Cytochrome P450 monooxygenases (CYPs) constitute a superfamily of heme-containing enzymes that are widely distributed among all biological kingdoms; they catalyze the hydroxylation of a wide variety of substrate molecules. CYP105s are the only CYP family that have been conserved with representatives in every Streptomyces species thus far investigated. Finally, we verified that CYP105P2 is a bacterial flavone hydroxylase, with potential for use as a biocatalyst. Our sequence analysis showed that CYP105P2 shares a high identity (92%) with CYP105P1 from S. avermitilis, and that it contains a dioxygen-binding region and a heme-iron-binding region, both of which are typical motifs of CYPs.

The structure of CYP105P2 from S. peucetius was determined at a resolution of 2.1 Å. It contains 15 α-helices and six β-strands. The putative active site of CYP105P2 is composed of a heme group and hydrophobic substrate-binding site. Although no exogenous ligands were added to the CYP105P2 protein during purification or crystallization, initial experimental maps indicated the presence of an unknown ligand near the active sites of both molecules in the asymmetric unit. A careful examination of the (Fo − Fc) difference density map following refinement indicated that there was a distinct electron density with a bent V-shape. The conformation of this density suggests that it could be interpreted as a biphenyl derivative, which was then fitted into this electron density map. A ligand resembling the biphenyl compound bisphenol A was unexpectedly found in the substrate-binding cavity; this ligand was probably incorporated during protein expression in E. coli. The bound ligand forms strong hydrophobic interactions with Pro82, Ala181, Met187, Leu189, Leu193, and Ile236 side-chains. In addition, the hydroxyl group of the biphenyl molecule forms hydrogen-bonding interactions with the NE2 of Gln177. Several hydrophobic residues (Pro82, Leu189, Leu193, and Ile236) in the hydrophobic ligand-binding cleft seem to be used invariantly to interact with various ligands.

>MSQPTAGAPAAPKARSCPFLPPDGIADIRAAAPVTRATFTSGHEAWLVTGYEQVRAVLRDPSFSVGVPHALHTQDGVVTQKPGRGSLLWQDAPEHTDDRKLLAKEFTVRRMQALRPNIQRIVDEHLDAIEARGGPVDLVKTFANPVPSMVISDLFGVPAERRAEFQEIAEAMMRVDQDAAATEAAGMRLGGLLYQLVQERRANPGDDLISALITTEDPDGVIDDMFLMNAAGTLLIAAHDTTACMIGLGTALLLDRPDQLALLQKDPSLIGNAVEELLRYLTIGQFGAERVATQDGEIGGVRIAKGEQVVTHLLSADFDPAFVEDPERFDITRRPAPHLAFGFGAHQCIGQQLARIELQIVFGTLFRRFPTLRLAKPVEELRFRNDMVFYGVHELPVTW[4x]> MKKNFFHLLIMLICSYISFAYANISDYRVMTWNLQGSSASTESKWNINVRQLLSGTAGVDILMVQEAGAIPTSAVRTGRHIQPFGVGIPIDEYTWNLGTTRRQDIRYIYYSPIDVGARRVNLAIVTRRRADNVYVLRPTTVASRPIIGIGLGNDVFLTTHALASGGPDAAAIVRVTYNFFRTPQMRHLSWLLGGDFNRAPDRLESDLMTEHLERLVTIIAPTEPTQIGGNILDYGVIVDRAPYSQRVEALRNPQLASDHYPVAFEAQHCG;> MKKLILLTLIIASFDIYAIDFVYRVDPNPPDVIFRDGFSLLGYNRDLQQLISGRSCAGGSSDSRYIVTTSDINKTYAIARAYYSHSKFKGNLYRYKIRADNNFYSLTPSVNYLESQGGHFNAYEKSMIRLQSEYVSTLSILPENIQKAVALVYDSSTGQIKDGTSTINTDYVSISSVSNPGVIPFLPEPQANTQQRIDAFGSLISSCFSIYSVCQTHRGQKTEVYKMPFYDARPVIQFIISGN;>[3x]MKKITSVCALLSLICSFNASAEWTGDYENIGYFSHEVISEFHVGQIDGGAYFCIKAVKADGSRSTPLIACSVSNESVWAPSFKVLLEQARYFYVTEQSVRIYYDHNVWTNQPFVNTFSTNALVGLSSCSAATDCFGPGKPKSKSKRDVEQ;>[2x]EWTGDSSINYYSDEVISDFHVGQFNRSAYFCIKTVKKSGEGTPIIACALSHDSKWIPSFNIMLEQARNFYITGHSIRVYVQPNVWSNKSFIEALSSNALVGLSSCSTSECFGPVKP

In this study, we identified and characterized a typhoid toxin-like A2B5 toxin, designated diarizonae toxin (DiaT), as a key virulence factor in Salmonella diarizonae. The DiaT genomic islet encodes two distinct B subunits, PltBd1 and PltBd2, which exhibit unique functional roles. Through genetic and functional analyses, we demonstrate that the heteropentameric assembly of PltBd1 and PltBd2 is essential for cytotoxicity, with our data suggesting PltBd1 facilitates toxin secretion and PltBd2 mediates host cell targeting. The holotoxin consists of a pentameric B subunit arrangement supporting a single PltA subunit, with the amphipathic C-terminal tail of PltA extending into the central pore formed by the B subunits.

To validate the structural insights from the cryo-EM map of the endogenously expressed DiaT holotoxin, we recombinantly expressed PltBd1 homopentameric holotoxin, PltBd2 homopentameric holotoxin, and PltBd1/PltBd2 heteropentameric holotoxin in E. coli. Cryo-EM analysis resolved these structures at resolutions of 3.05 Å, 2.61 Å, and 2.94 Å, respectively. Additionally, recombinant co-expression of PltBd1, PltBd2, PltA, and CdtB in Escherichia coli similarly demonstrated the presence of the heteropentameric holotoxin (S1G). Notably, the heteropentameric holotoxin purified from E. coli exhibited an identical composition and assembly to the endogenous DiaT holotoxin purified from S. diarizonae. Structural analysis confirmed consistent and distinct amino acid differences that enable the differentiation of PltBd1 and PltBd2 in the endogenous DiaT holotoxin, further reinforcing their reliability as markers for B subunit identification. Three tightly packed PltBd1 subunits were connected with dimeric PltBd2 subunits to form the heteropentamer in the holotoxin structure. The stronger hydrophobic interactions between PltBd2 and PltA, along with additional polar interactions involving PltBd1 and PltA, establish a finely balanced assembly that facilitates the stable accommodation of PltA’s C-terminal tail by the heteropentameric B subunits. Although PltBd1 and PltBd2 can individually form homopentamers, the heteropentamer is preferentially selected by PltA, likely due to its enhanced structural compatibility and complementary interactions. All holotoxins demonstrated cytotoxic activity, but the PltBd2 homopentamer exhibited the highest potency, approximately threefold greater than the PltBd1/PltBd2 heteropentameric toxin (DiaT) and nearly 75-fold greater than the PltBd1 homopentamer.(3-{(1R)-3-(3,4-dimethoxyphenyl)-1-[({(2S)-1-[(2S)-2-(3,4,5-trimethoxyphenyl)pent-4-enoyl]piperidin-2-yl}carbonyl)oxy]propyl}phenoxy)acetic acid | C39 H47 N O11 | 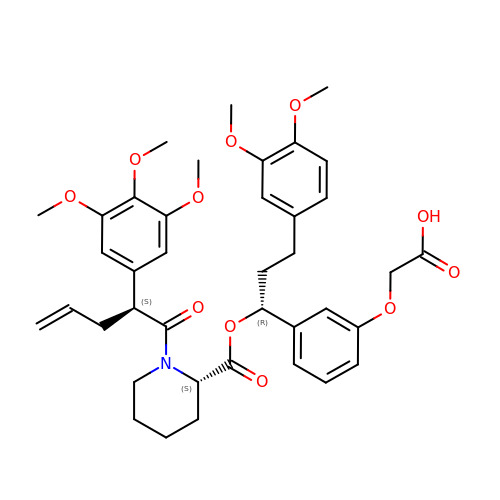GTVAUHXUMYENSK-RWSKJCERSA-N>MADSTTPGYTVVKNDWKKAVKQLQDGLKNKTISTIKVSFNGNSVGEVTPASSGAKKADRDAAAEKLYNLVNTQLDKLGDGDYVDFEVTYNLATQIITKAEAEAVLTKLQQYNDKVLINSATDTVKGMVSDTQVDSKNVAANPLKVSDMYTIPSAITGSDDSGYSIAKPTEKTTSLLYGTVGDATAGKAITVDTASNEAFAGNGKVIDYNKSFKATVQGDGTVKTSGVV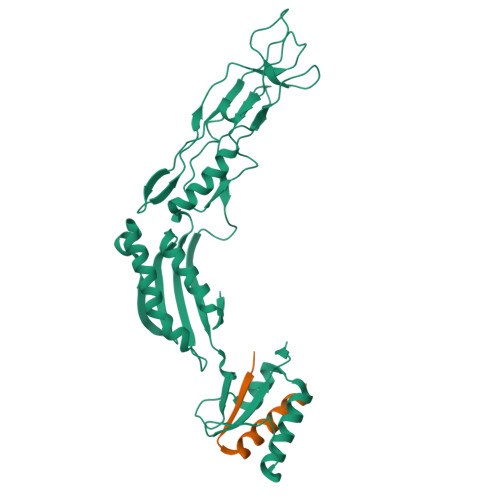LKDASDMAATGTIKVRVTSAKEESIDVDSSSYISAENLAKKYVFNPKEVSEAYNAIVALQNDGIESDLVQLVNGKYQVIFYPEGKRLETKS[2x];> MADIIADADSPAKITIKANKLKDLKDYVDDLKTYNNTYSNVVLEHHHHHH> QPRKKRPEDFKFGKILGEGSFSTVVLARELATSREYAIKILEKRHIIKENKVPYVTRERDVMSRLDHPFFVKLYFTFQDDEKLYFGLSYAKNGELLKYIRKIGSFDETCTRFYTAEIVSALEYLHGKGIIHRDLKPENILLNEDMHIQITDFGTAKVLSPESKQARANSFVGTAQYVSPELLTEKSACKSSDLWALGCIIYQLVAGLPPFRAGNEYLIFQKIIKLEYDFPEKFFPKARDLVEKLLVLDATKRLGCEEMEGYGPLKAHPF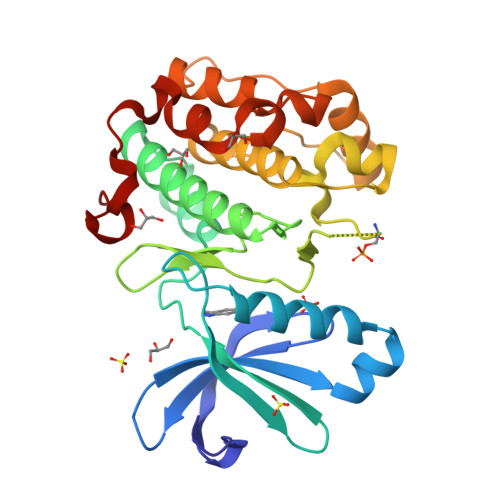FESVTWENLHQQTPPKL>HPETLVKVKDAEDQLGARVGYIELDLNSGKILESFRPEERFPMMSTFKVLLCGAVLSRIDAGQEQLGRRIHYSQNDLVEYSPVTEKHLTDGMTVRELCSAAITMSDNTAANLLLTTIGGPKELTAFLHNMGDHVTRLDRWEPELNEAIPNDERDTTMPVAMATTLRKLLTGELLTLASRQQLIDWMEADKVAGPLLRSALPAGWFIADKSGAGERGSRGIIAALGPDGKPSRIVVIYTTGSQATMDERNRQIAEIGASLIKHW[2x];>AGVMTGAKFTQIQFGMTRQQVLDIAGAENCETGGSFGDSIHCRGHAAGDYYAYATFGFTSAAADAKVDSKSQEKLLAPSAPTLTLAKFNQVTVGMTRAQVLATVGQG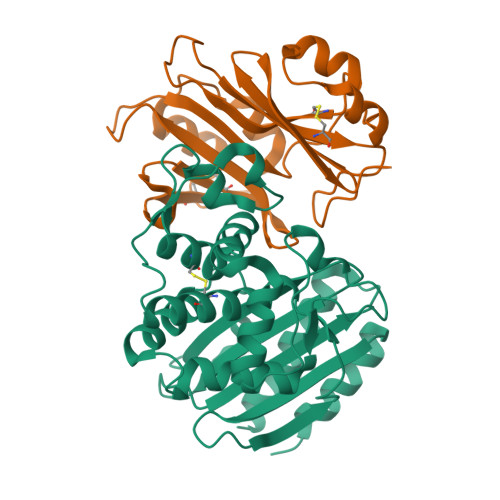SCTTWSEYYPAYPSTAGVTLSLSCFDVDGYSSTGFYRGSAHLAFTDGVLQGKRQWDLV[2x]>MTEEKIEEARQSIKEAERSLREGNPEKALDAVARALSLVNELERLARKTGSTEVLIEAARLAIEVARVALKVGSPEMAQLAVELALRLVQELERQARKTGSTEVLIEAARLAIEVARVAFKVGSPETAREAARTALELVEELERQARKTGSEEVLERAARLAEEVARVAEEIGDPELARKAMKVAIRLTEELLKKSLRELRRILEELKEMLERLEKNPDKDVIVKVLKVIVKAIEASVENQRISADNQRALARLAGSWSGGGSEQK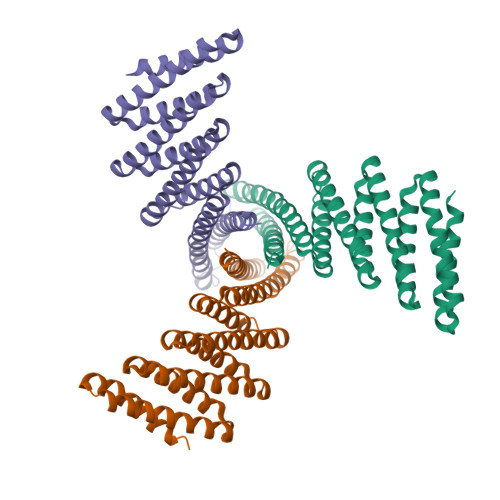LISEEDLGGS[3x]> GDVEEAIERAVVHVADTMRSGPSNSASVPALTAVETGHTSQVTPSDTMQTRHVKNYHSRSESTVENFLGRSACVYMEEYKTTDNDVNKKFVAWPINTKQMVQMRRKLEMFTYLRFDMEVTFVITSRQDPGTTLAQDMPVLTHQIMYVPPGGPIPAKVDDYAWQTSTNPSIFWTEGNAPARMSIPFISIGNAYSNFYDGWSNFDQRGSYGYNTLNNLGHIYVRHVSGSSPHPITSTIRVYFKPKHTRAWVPRPPRLCQYKKAFSVDFTPTPITDTRKDINTVT;> SDRVRSITLGNSTITTQECANVVVGYGRWPTYLRDDEATAEDQPTQPDVATCRFYTLDSIKWEKGSVGWWWKFPEALSDMGLFGQNMQYHYLGRAGYTIHVQCNASKFHQGCLLVVCVPEAEMGGAVVGQAFSATAMANGDKAYEFTSATQSDQTKVQTAIHNAGMGVGVGNLTIYPHQWINLR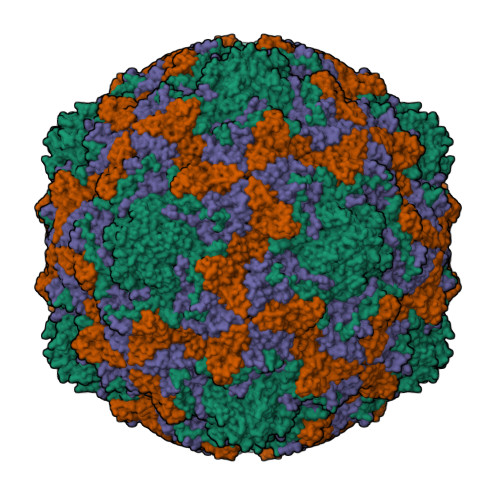TNNSATIVMPYINSVPMDNMFRHYNFTLMVIPFVKLDYADTASTYVPITVTVAPMCAEYNGLRLAQ;> LPTMNTPGSTQFLTSDDFQSPCALPQFDVTPSMNIPGEVKNLMEIAEVDSVVPVNNVQDTTDQMEMFRIPVTINAPLQQQVFGLRLQPGLDSVFKHTLLGEILNYYAHWSGSMKLTFVFCGSAMATGKFLIAYSPPGANPPKTRKDAMLGTHIIWDIGLQSSCVLCVPWISQTHYRLVQQDEYTSAGYVTCWYQTGMIVPPGTPNSSSIMCFASACNDFSVRMLRDTPFISQDNKL;> GAQVSTQKTGAHETSLSAAGNSIIHYTNINYYKDAASNSANRQDFTQDPSKFTEPVKDVMIKSLPAL Here we describe the molecular basis of the reaction mechanism and dual NADH/NADPH-specificity of D2HDH, a 2-hydroxyacid dehydrogenase from the extreme halophile Haloferax mediterranei, an organism whose proteins have to remain active in high intracellular concentrations of KCl. Sequence analysis has identified D2HDH as a member of the DDH clade of the D-isomer specific 2-hydroxyacid dehydrogenase enzyme family (2HADH), which has potential applications in the synthesis of chiral fine chemicals including alcohols, and hydroxy or amino acids from ketones or ketoacids. Structural studies have shown that all members of this family share a common fold based on two domains, which cycle between open and closed conformational states that serve to close the inter-domain cleft, bringing the substrates together during catalysis. The D2HDH dimer has an overall ellipsoidal appearance in which each monomer is folded into two domains (d1; residues 1–92 and 283–308 and d2; residues 93–282).

Thus far, to our knowledge, no structures of the wider DDH family have been determined with a reduced hydroxy acid substrate. To better understand the mode of product recognition by D2HDH, we attempted to grow crystals of a non-productive ternary complex of the enzyme with a variety of 2-hydroxyacids (including 2-hydroxyhexanoic acid) and NAD(P)H, to complement the 2-ketoacid structures described above, but the crystals that were obtained were of poor quality, and not suitable for structure determination. Under these crystallization conditions the enzyme would be expected to turn over the substrates leading to crystals that might contain a mixture of oxidised and reduced components. Given that the equilibrium constant favours the production of the reduced substrate, reaction turnover would lead to significant oxidation of the NAD(P)H to NAD(P)+ and the concomitant accumulation of mM concentrations of D-2-hydroxyhexanoic acid, albeit in a mixture with unreacted ketoacid in excess compared to the protein concentration (~0.1 mM). In this structure the refined electron density was planar for the nicotinamide ring consistent with the major component bound at the active site being the oxidised cofactor. Although the electron density for the substrate was clear, it could not be explained by either a ketoacid or a D-2-hydroxyacid alone. For example, fitting the density with a ketoacid left a significant additional bulge close to the substrate C2, particularly for subunit B. This suggested that a mixture of reduced and oxidised substrate was present. Careful refinement of this structure showed that the substrate density could be best explained as a 2:1 mixture of 2-ketohexanoic acid in the abortive orientation and D-2-hydroxyhexanoic acid in a productive orientation.

>MHIERLAVDESVGRAMPPQRFIEALSDLGVPVEFAGEDEQFGPGDAVASFGHRDAFLDADWVHCIRAGYDEFPVGVYEEAGTYLTNSTGIHGTTVGETVAGYMLTFARRLHAYRDAQHDHAWDLPRYEEPFTLAGERVCVVGLGTLGRGVVDRAAALGMEVVGVRRSGDPVDNVSTVYTPDRLHEAIADARFVVLATPLTDETEGMVAAPEFETMREDASLVNVARGPVVVESDLVAALDSGDIAGAALDVFSEEPLPEDSPLWDFEDVLITPHVSAATSKYHEDVAALIRENIEKIATGDELTNRVV[2x]> TGDDKSDEWKKNEWNNWLIKTEEDWKLFNTAVENKKNRWLEKRDKELEVWLMNMQNRWLHYRENEENEYKAEAMKNSATWDDSQWEQWIKTEGKKGMEADLKKWLNDKETFLDGWISKEWVQWKNERMLQWLSVDWKHKEDETFEHYKSSKFTNVLHIKKKKKWTKWKERTNKEKEEWNNWVKGKENLYVNNKWDKWLKWKKDKRALYSQKFLTFINKWISDKQWTVWIEDQGGSTLGTKHHHHHH

Tryptophan Rich Antigens (TRAgs) are encoded by a multi-gene family found in all Plasmodium species, but are significantly expanded in P. vivax and closely related parasites. Potential candidate proteins include the Tryptophan rich antigen multi-gene family (TRAgs), which all share a Tryptophan-Threonine-rich domain of unknown function (PFAM ID PF12319, OrthoMCL ID OG6_145873), usually at their C-terminus. We show that multiple P. vivax TRAgs are expressed on the merozoite surface and that one, PVP01_0000100 binds red blood cells with a strong preference for reticulocytes. Using X-ray crystallography, we solved the structure of the PVP01_0000100 C-terminal tryptophan rich domain, which defines the TRAg family, revealing a three-helical bundle that is conserved across Plasmodium and has structural homology with lipid-binding BAR domains involved in membrane remodelling.

To establish how the C-terminal Tryptophan/Threonine-rich domain of PVP01_0000100 mediates reticulocyte binding we used X-ray crystallography to experimentally determine the structure of this domain. The structure was refined to 1.45 Å resolution and had one molecule in the asymmetric unit. Consistent with the NetSurfP predictions, the structure is composed primarily of α-helices that are arranged into an extended three-helical bundle with small helical domains at each end. The conserved tryptophan residues that define the domain are distributed along the length of the helical bundle and are all buried within the fold, contributing to the arrangement of the long helices. Since experimental determination of this structure, new methods for prediction of 3D protein structures have been accelerated through use of deep-learning strategies as exemplified by AlphaFold2 (AF2). AF2 predictions of the PVP01_0000100 Tryptophan/Threonine-rich domain structure closely resemble the structure we experimentally determined, with an RMSD of 1.56 Å over 213 Cα atoms. Analysis of the surface charge of the PVP01_0000100 revealed extended positively charged patches, mainly on the N- terminal and concave side of the protein surface, similar to the shape and surface charge of BAR domains, suggesting a potential lipid binding function. PVP01_0000100 CTD showed specific and strong binding to sulfatide, an anionic glycosphingolipid found on the outer leaflet of multiple cell types, including red blood cells. PVP01_0000100 binding to sulfatide followed a sigmoidal binding curve, suggesting a saturable and hence specific interaction.> MTFRYRGPSPKGDQPKAIAGLVEALRDGERFVTLLGATGTGKTVTMAKVIEALGRPALVLAPNKILAAQLAAEFRELFPENAVEYFISYYDYYQPEAYVPGKDLYIEKDASINPEIERLRHSTTRSLLTRRDVIVVASVSAIYGLGDPREYRARNLVVERGKPYPREVLLERLLELGYQRNDIDLSPGRFRAKGEVLEIFPAYETEPIRVELFGDEVERISQVHPVTGERLRELPGFVLFPATHYLSPEGLEEILKEIEKELWERVRYFEERGEVLYAQRLKERTLYDLEMLRVMGTCPGVENYARYFTG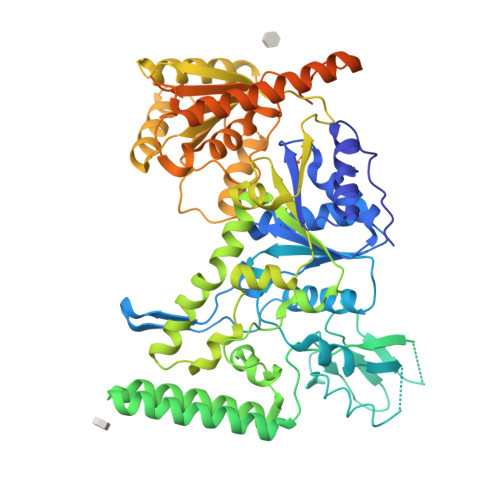KAPGEPPYTLLDYFPEDFLVFLDESHVTVPQLQGMYRGDYARKKTLVDYGFRLPSALDNRPLRFEEFLERVSQVVFVSATPGPFELAHSGRVVEQIIRPTGLLDPLVRVKPTENQILDLMEGIRERAARGERTLVTVLTVRMAEELTSFLVEHGIRARYLHHELDAFKRQALIRDLRLGHYDCLVGINLLREGLDIPEVSLVAILDADKEGFLRSERSLIQTIGRAARNARGEVWLYADRVSEAMQRAIEETNRRRALQEAYNLEHGITPETVRKEVRAVIRPEGYEEAPLEADLSGEDLRERIAELELAMWQAAEALDFERAARLRDEIRALEARLQGVRAPEPVPGGRKRKRR> MKDSGDSKDQQLMVALRVRPISVAELEEGATLIAHKMDEQMVVLMDPMEDPDDILRAHRSREKSYLFDVAFDFTATQEMVYQATTKSLIEGVISGYNATVFAYGPTGCGKTYTMLGTDHEPGIYVRTLNDLFRAIEETSNDMEYEVSMSYLEIYNEMIRDLLNPALGYLELREDSKGVIQVAGITEVSTINAKEIMQLLMKGNRQRTQEPTAANQTSSRSHAVLQVAVRQRSRVKNILQEVRQGRLFMIDLAGSERASQTQNRGQRMKEGAHINRSLLALGNCINALSDKGSNKYINYRDSKLTRLLKDSLGGNSRTVMIAHISPASTAFEESRNTLTYAGRAKNIRTRVKQN

KIF19A, a kinesin-8 sub-family member, is unique in that it possesses both functions, MT-based active motility toward the plus-end and MT depolymerizing activity. We recently reported that KIF19A functions as a MT-depolymerizing kinesin in the control of cilium length. Thus, to elucidate the molecular mechanism of the dual KIF19A functions, we performed crystal structure analysis of the mouse KIF19A motor domain as well as cryo-electron microscopy (cryo-EM) reconstruction of the KIF19A motor domain complexed with a MT. In the catalytic core of KIF19A, the KIF19A-specific feature of adopting two different interfaces for MTs and tubulins is utilized to achieve the dual functions.

We investigated the molecular mechanism of the dual functions of the KIF19A 353WT monomeric motor by solving its crystal structure at 2.7 Å resolution. At the initial stage of the 353WT structure determination process, the residues of the switch II helix α4 could not be determined because there was no corresponding density at the site where α4 is usually located at the center of the MT-binding interface. Instead, we found an unmodeled helical-like density, which was more distant from the KIF19A catalytic core. When the Cys283 residue was assigned to this anomalous signal, all the residues in α4 and the following loop L12 were reasonably determined. The overall structure of the KIF19A 353WT motor domain shared a similar triangle-shape with other kinesins, which consists of a central β-sheet of eight strands, sandwiched between six α-helices, three on either side. In the 353WT atomic structure, Mg2+-ADP was found embedded in the nucleotide-binding pocket. In comparison with previously solved motor domains of various KIFs, the remarkable features of the KIF19A motor domain are concentrated on its MT-binding side and include the long and wide L2 loop, the flexible L8 loop, the disordered α4 helix, and the short α6 helix. Loop L2 is located at the minus-end side (rear side) of the MT-binding surface and is atypically long. Loop L8, which is the major MT-binding region at the plus-end side, is more retracted toward the catalytic core compared with that of kinesin-13. The switch II helix α4, which is considered the main contributor to MT-based kinesin motility, is more distant from the motor domain than those of other kinesins including kinesin-8 KIF18A.2-[(5-nitro-1H-benzimidazol-2-yl)sulfanyl]-N-(4-phenoxyphenyl)acetamide 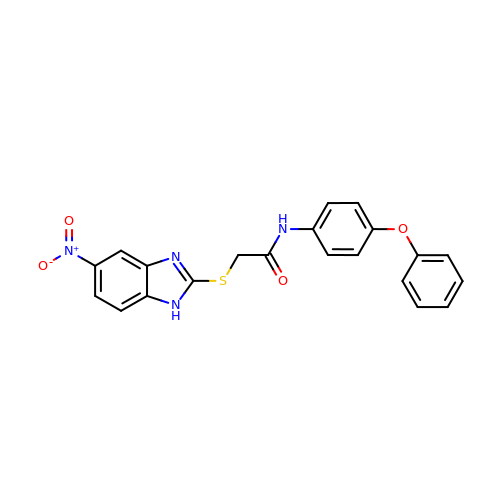| C21 H16 N4 O4 S | IPZUVKDSPDAHMB-UHFFFAOYSA-N> SMFEFDNLAPMLATHGTVAGLKASQWAFEGMWDGYRLLVEADHGAVRLRSRSGRDVTAEYPQLRALAEDLADHHVVLDGEAVVLDSSGVPSFSQMQNRGRDTRVEFWAFDLLYLDGRALLGTRYQDRRKLLETLANATSLTVPELLPGDGAQAFACSRKHGWEGVIAKRRDSRYQPGRRCASWVKDKHWNTQEVVIGGWRAGEGGRSSGVGSLLMGIPGPGGL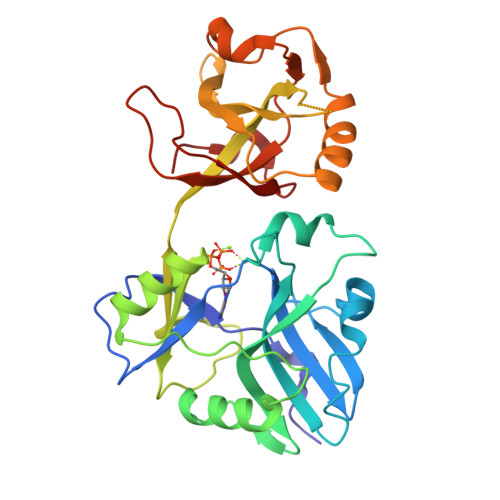QFAGRVGTGLSERELANLKEMLAPLHTDESPFDVPLPARDAKGITYVKPALVAEVRYSEWTPEGRLRQSSWRGLRPDKKPSEVVRE> MLNQELELSLNMAFARAREHRHEFMTVEHLLLALLSNPSAREALEACSVDLVALRQ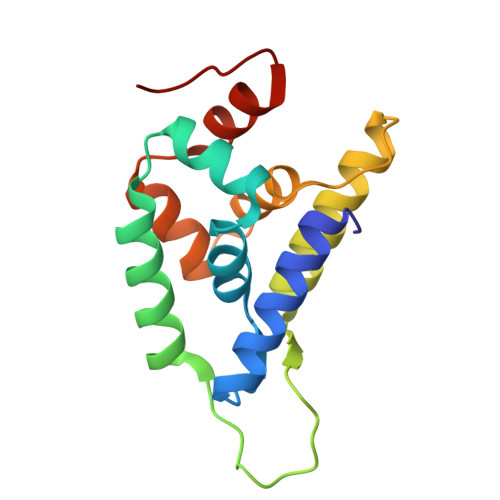ELEAFIEQTTPVLPASEEERDTQPTLSFQRVLQRAVFHVQSSGRNEVTGANVLVAIFSEQESQAAYLLRKHEVSRLDVVNFISHGTRKDE BETA-D-ERYTHROFURANOSYL-ADENOSINE | 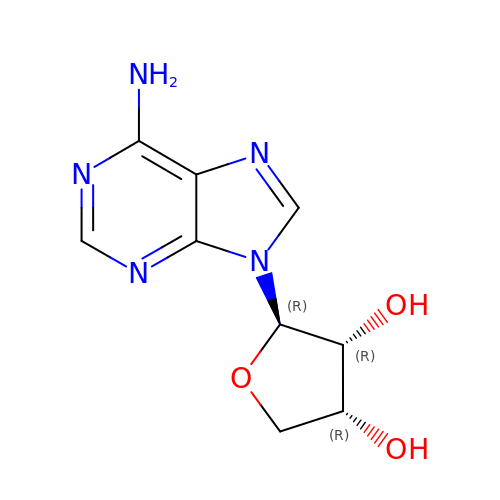C9 H11 N5 O3 | DTGVOXMKTYPSSO-NVMQTXNBSA-N> MPSYKSSRVLVRDVPEELVD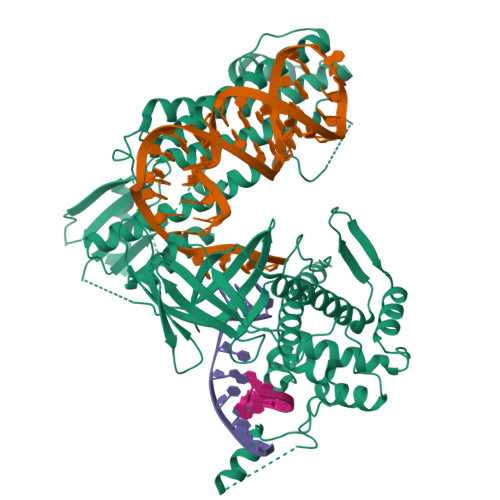HYERSHRVAAFFMRLLLAMRREPYSLRMRDGTEREVDLDETDDFLRSAGCEEPDAVSDDLRSFALAVLHQDNPKKRAFLKSENCVSILCLEKSASGTRYYKRPGYQLLKKAIEEEWGWDKFEASLLDERTGEVAEKFAALSMEDWRRFFAARDPDDLGRELLKTDTREGMAAALRLRERGVFPVSVPEHLDLDSLKAAMASAAERLKSWLACNQRAVDEKSELRKRFEEALDGVDPEKYALFEKFAAELQQADYNVTKKLVLAVSAKFPATEPSEFKRGVEILKEDGYKPLWEDFRELGFVYLAERKWERRRGGAAVTLCDADDSPIKVRFGLTGRGRKFVLSAAGSRFLITVKLPCGDVGLTAVPSRYFWNPSVGRTTSNSFRIEFTKRTTENRRYVGEVKEIGLVRQRGRYYFFIDYNFDPEEVSDETKVGRAFFRAPLNESRPKPKDKLTVMGIDLGINPAFAFAVCTLGECQDGIRSPVAKMEDVSFDSTGLRGGIGSQKLHREMHNLSDRCFYGARYIRLSKKLRDRGALNDIEARLLEEKYIPGFRIVHIEDADERRRTVGRTVKEIKQEYKRIRHQFYLRYHTSKRDRTELISAEYFRMLFLVKNLRNLLKSWNRYHWTTGDRERRGGNPDELKSYVRYYNNLRMDTLKKLTCAIVRTAKEHGATLVAMENIQRVDRDDEVKRRKENSLLSLWAPGMVLERVEQELKNEGILAWEVDPRHTSQTSCITDEFGYRSLVAKDTFYFEQDRKIHRIDADVNAAINIARRFLTRYRSLTQLWASLLDDGRYLVNVTRQHERAYLELQTGAPAATLNPTAEASYELVGLSPEEEELAQTRIKRKKREPFYRHEGVWLTREKHREQVHELRNQVLALGNAKIPEIRT> MMGSSHHHHHHHHHSSGENLYFQGGSMIEVTEVSIAELRDALESGRTTAVELVQAYLARIDAYDAPGTPTALNAVVVRNPDALAEAQASDARRARGEPLGPLDGIPYTAKDSYLVKGLTAASGSPAFKDLVAQRDAFTVERLRAAGAICLGKTNMPPMANGGMQRGVYGRAESPYNAAYLTAPFASGSSNGAGTATAASFAAFGLAEETWSSGRGPASNNGLCAYTPSRGVISVRGNWPLTPTMDVVVPYARSMADLLEILDVVVADDPDTRGDLWRMQPWVPIPKASEVRPASYPALAAGAEALAGKRFGVPRMFINADPDAGTSESPGIGGPTGQRIHTRPSVIALWEQARKALEAAGAEVIEVDFPLVSNCEGDRPGAPTVFNRGLVSKEFLHDELWELSAWGFDDFLRANGDPKLNRL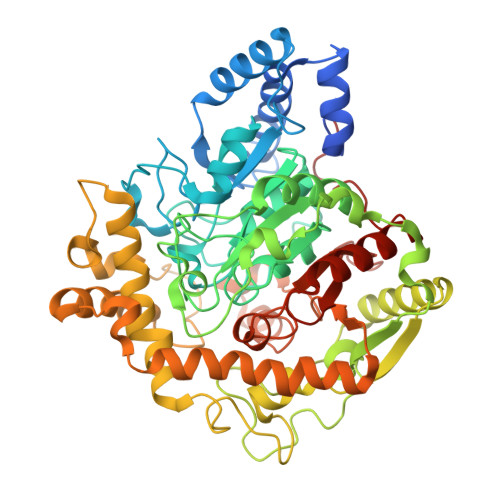ADVDGPQIFPHDPGTLPNREGDLAAGMDEYVRMAERGIKPWDRIATLPDGLRGLEETRRIDLEEWMRRLRLDAVLFPTVADVGPADADVNPASADIAWSNGVWVANGNLAIRHLGVPTVTVPMGVMADIGMPVGLTFAGRAYDDSALLRFAAAFESTGSRRIVPPRTPPLASK>APQVVDKVAAVVNNGVVLESDVDGLMQSVKLNAAQARQQLPDDATLRHQIMERLIMDQIILQMGQKMGVKISDEQLDQAIANIAKQNNMTLDQMRSRLAYDGLNYNTYRNQIRKEMIISEVRNNEVRRRITILPQEVESLAQQVGNQNDASTELNLSHILIPLPENPTSDQVNEAESQARAIVDQARNGADFGKLAIAHSADQQALNGGQMGWGRIQELPGIFAQALSTAKKGDIVGPIRSGVGFHILKVNDLRGESKNISAAQKDRAYRMLMNRKFSEE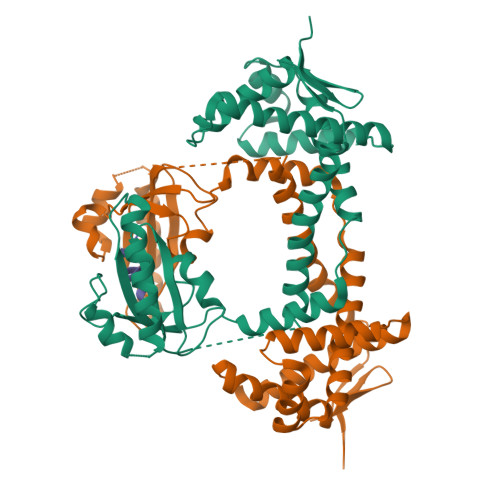AASWMQEQRASAYVKILSN[2x];> NFTLKFWDIFRK>[2x]PVPRNYNYYQAPEKRSKHIMPS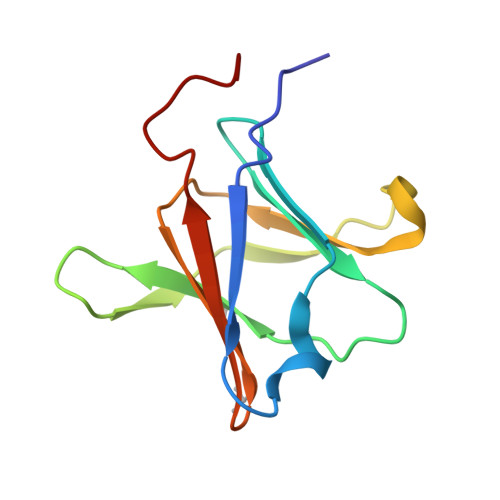EIFDDGTFTYFGFKNITLQPAIFVVQPDGKLSMTDAAIDPNMTNSGLRWYRVNEIAEKFKLIKDKALVTVINKGYGKNPLT>[2x]GAKMNESDIWFEEKLQEVECEEQRLRKLHAVVETLVNHRKELALNTAQFAKSLAMLGSSEDNTALSRALSQLAEVEEKIEQ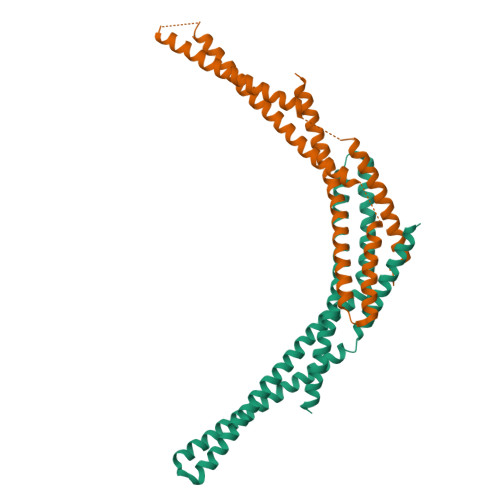LHQEQANNDFFLLAELLSDYIRLLAIVRAAFDQRMKTWQRWQDAQATLQKKREAEARLLWANKPDKLQQAKDEILEWESRVTQYERDFERISTVVRKEVIRFEKEKSKDFKNHVIKYLETLLYSQQQLAKYWEAFLPEAKAIS>[2x]SKTKPFSLPSLTLDELSNSRFPAPIVQLYTNPHDNLVVQPQNGRCTIDGLLQGTTQLVSCNVCSFRGTLGDGQPASHSEEEIMPMA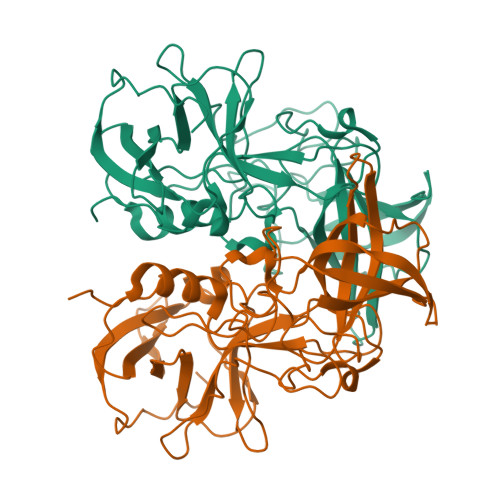FNIQREIMLENLDGSPYDPTDDIPAVLGSPDFQGVVFGILSQRNTDGQTRAHEAKVDTRLARFAPKLGFVVATVENTDFHANQPCRFTPVGLGGDNNRDFNQWGLPAYGGALTNNTNLAPPVMPVYPGEQLLFFRSQLPSSGGVVGGWLDCLLPQEWVQHFFQESATSQSDVALVRYINPTTGRVLFEAKLHKQGFLTVAASGSYPLVVPADGYFRFESWVNQFYTLAPMGNGSG> APTAPSIDMYGSNNLQFSKIELAMETTSGYNDMVKYHELAKIKVKFNQWSGTSGDTYNVYFDGVKVATGAITGSQTTASFEYGQGGLYQMEIEACDATGCSKSAPVEITIADTDGSHLKPLTMNVDPNNKSYNTDPSIVMGTYFVEWGIYGRDYTVDNMPVDNLTHILYGFIPICGPNESVKSVGGNSFNALQTACRGVNDYEVVIHDPWAAYQKSFPQAGHEYSTPIKGNYAMLMALKQRNPDLKIIPSIGGGTLSDPFYDFVDKKNRDTFVASVKKFLKTWKFYDGVDIDWEFPGGGGAAADKGDPVNDGPAYIALMRELRVMLDELEAETGRTYELTSAIGVGYDKIEDVDYADAVQYMDYIFAMTYDFYGGWNNVPGHQTALYCGSFMRPGQCDGGGVDENGEPYKGPAYTADNGIQLLLAQGVPANKLVLGTAMYGRGWEGVTPDTLTDPNDPMTGTATGKLKGSTAQGVWEDGVIDYKGIKSFMLGANNTGINGFEYGYDAQAEAP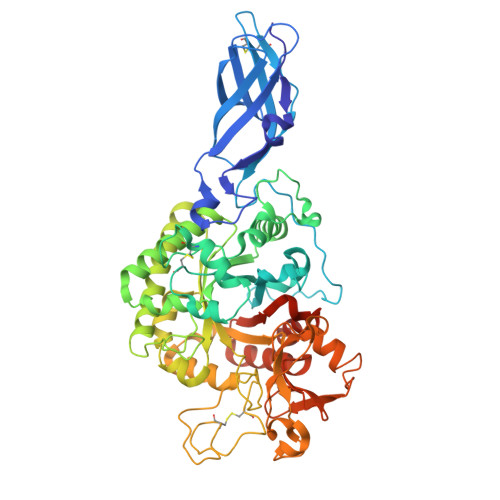WVWNRSTGELITFDDHRSVLAKGNYAKSLGLAGLFSWEIDADNGDILNAMHEGMAGGVVTPPNRRSHHHHHH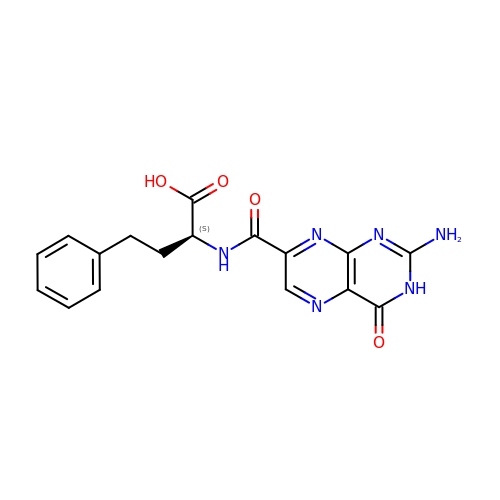(2S)-2-[(2-azanyl-4-oxidanylidene-3H-pteridin-7-yl)carbonylamino]-4-phenyl-butanoic acid | C17 H16 N6 O4 | CHPGDIWMRACXGP-JTQLQIEISA-N>MTSATASFATRTSLAADLAALGLAWGDAIMVHAAVSRVGRLLDGPDTIIAALRDTVGPGGTVLAYADWEARYEDLVDDAGRVPPEWREHVPPFDPQRSRAIRDNGVLPEFLRTTPGTLRSGNPGASLVALGAKAEWFTADHPLDYGYGEGSPLAKLVEAGGK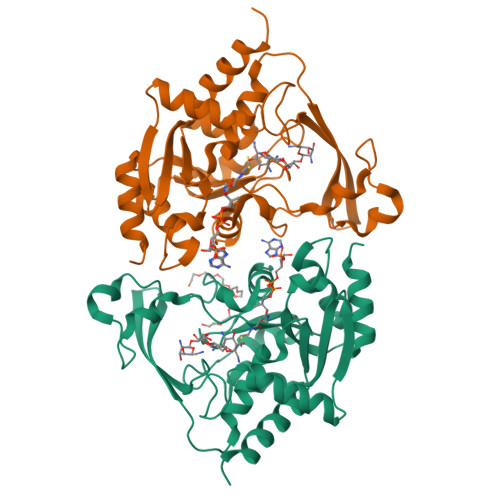VLMLGAPLDTLTLLHHAEHLADIPGKRIKRIEVPFATPTGTQWRMIEEFDTGDPIVAGLAEDYFAGIVTEFLASGQGRQGLIGAAPSVLVDAAAITAFGVTWLEKRFGTPSP[4x]> MIVRNLGDIRKTDRNVRSDGWASARMLLKDDGMGFSFHVTTLFAGSELRMHYQNHLEAVLVLKGTGTIEDLATG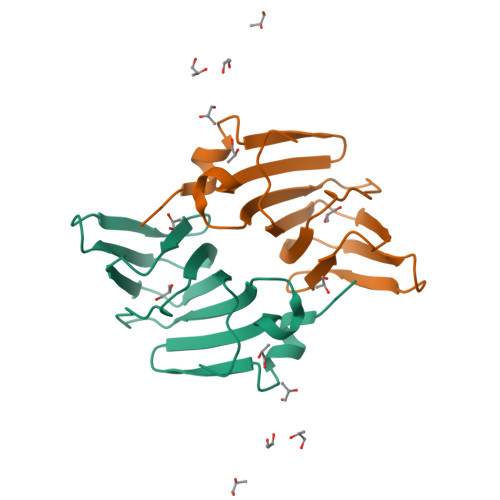EVHALRPGVMYALDDHDRHIVRPETDILTACVFNPPVTGREVHDESGAYPADPELAREPVAADNWSHPQFEK>[7x]ASWSHPQFEKAGFSRHNRDTSAP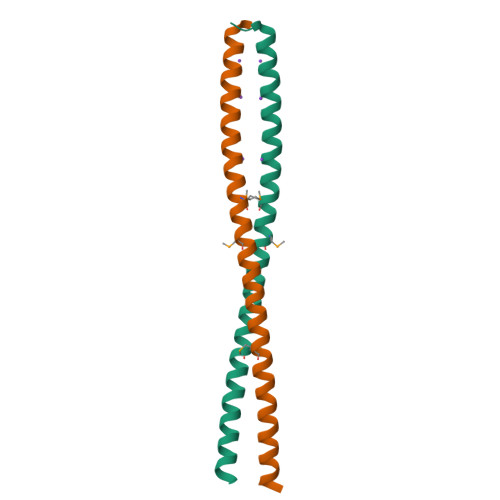ANFASSSTLEKRIEDLEKEVLRERQENLRLTRLMQDKEEMIGKLKEEIDLLNRDLDDMEDENEQLKQENKTLLKVVGQLTR>[4x]MAKKTSSGRGKLPPGPTPLPVIGNILQIDIKDVSKSLTNLSKIYGPVFTLYFGLERMVVLHGYEVVKEALIDLGEEFSGRGHFPLAERANRGFGIVFSNGKRWKEIRRFSLMTLRNFGMGKRSIEDRVQEEARCLVEELR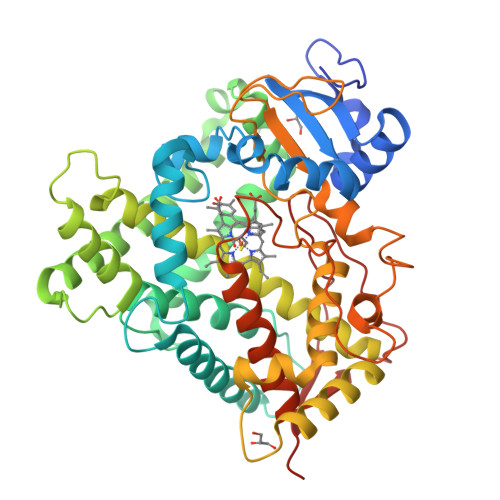KTKASPCDPTFILGCAPCNVICSIIFQKRFDYKDQQFLNLMEKLNENIRIVSTPWIQICNNFPTIIDYFPGTHNKLLKNLAFMESDILEKVKEHQESMDINNPRDFIDCFLIKMEKEKQNQQSEFTIENLVITAADLLGAGTETTSTTLRYALLLLLKHPEVTAKVQEEIERVVGRNRSPCMQDRGHMPYTDAVVHEVQRYIDLIPTSLPHAVTCDVKFRNYLIPKGTTILTSLTSVLHDNKEFPNPEMFDPRHFLDEGGNFKKSNYFMPFSAGKRICVGEGLARMELFLFLTFILQNFNLKSLIDPKDLDTTPVVNGFASVPPFYQLCFIPIHHHH>AMGSGVLPRPCRVLVLLNPRGGKGKALQLFRSHVQPLLAEAEISFTLMLTERRNHARELVRSEELGRWDALVVMSGDGLMHEVVNGLMERPDWETAIQKPLCSLPAGSGNALAASLNHYAGYEQVTNEDLLTNCTLLLCRRLLSPMNLLSLHTASGLRLFSVLSLAWGFIADVDLESEKYRRLGEMRFTLGTFLRLAALRTYRGRLAYLPVGRVGSKTPASPVVVQQGPVDAHLVPLEEPVPSHWTVVPDEDFVLVLALLHSHLGSEM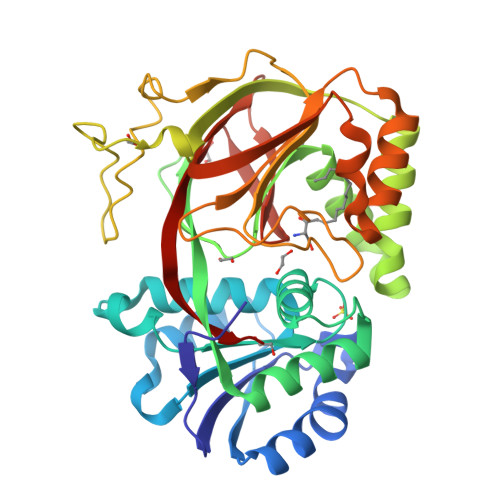FAAPMGRCAAGVMHLFYVRAGVSRAMLLRLFLAMEKGRHMEYECPYLVYVPVVAFRLEPKDGKGVFAVDGELMVSEAVQGQVHPNYFWMVSG[3x]> ASTEEKWARLARRIAGAGGVTLDGF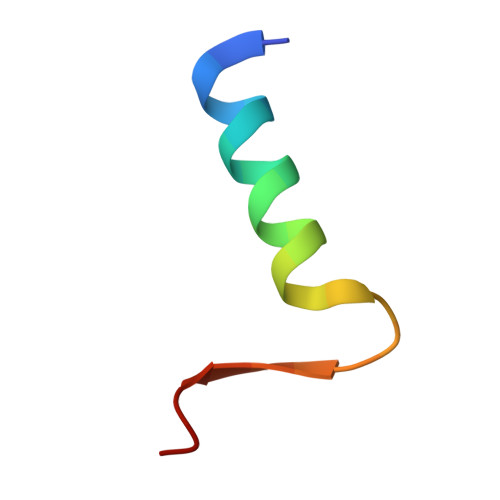G>KKKILITWPLPEAAMARARESYDVIAHGDDPKITIDEMIETAKSVDALLITLNEKCRKEVIDRIPENIKCISTYSIGFDHIDLDA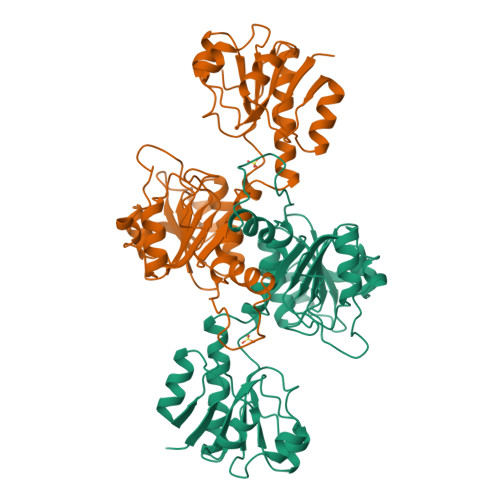CKARGIKVGNAPHGVTVATAEIAMLLLLGSARRAGEGEKMIRTRSWPGWEPLELVGEKLDNKTLGIYGFGSIGQALAKRAQGFDMDIDYFDTHRASSSDEASYQATFHDSLDSLLSVSQFFSLNAPSTPETRYFFNKATIKSLPQGAIVVNTARGDLVDNELVVAALEAGRLAYAGFDVFAGEPNINEGYYDLPNTFLFPHIGSAATQAREDMAHQANDLIDALFGGADMSYALA[2x]(1r,2R,3S,4r,5R,6S)-4-hydroxy-2,3,5,6-tetrakis(phosphonooxy)cyclohexyl trihydrogen diphosphate 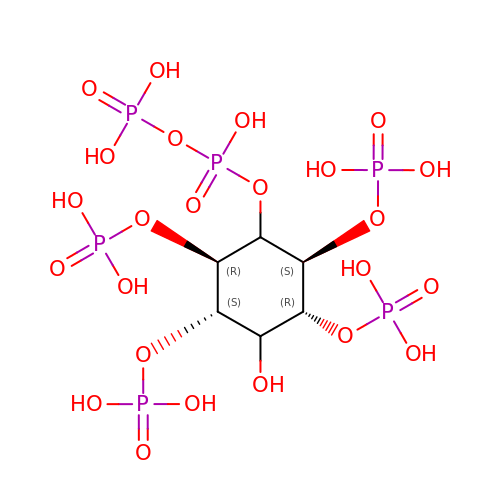| C6 H18 O24 P6 | FFZGWHDHUIRNPY-KXXVROSKSA-N> ETDEEPEEPGTTGSFVEMVDNLRGKSGQGYYVEMTVGSPPQTLNILVD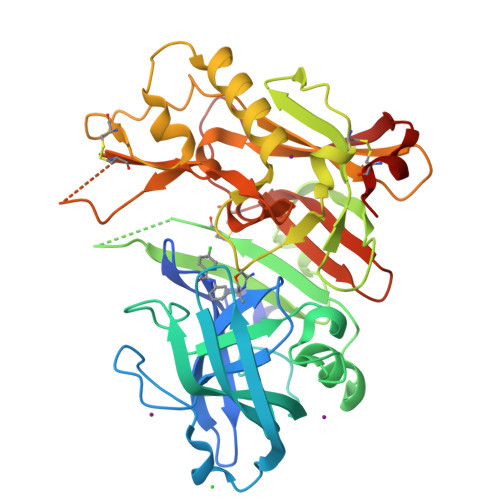TGSSNFAVGAAPHPFLHRYYQRQLSSTYRDLRKGVYVPYTQGKWEGELGTDLVSIPHGPNVTVRANIAAITESDKFFINGSNWEGILGLAYAEIARPDDSLEPFFDSLVKQTHVPNLFSLQLCGAGFPLNQSEVLASVGGSMIIGGIDHSLYTGSLWYTPIRREWYYEVIIVRVEINGQDLKMDCKEYNYDKSIVDSGTTNLRLPKKVFEAAVKSIKAASSTEKFPDGFWLGEQLVCWQAGTTPWNIFPVISLYLMGEVTNQSFRITILPQQYLRPVEDVATSQDDCYKFAISQSSTGTVMGAVIMEGFYVVFDRARKRIGFAVSACHVHDEFRTAAVEGPFVTLDMEDCGYN5-[(diaminomethylidene)amino]-2-oxopentanoic acid | C6 H11 N3 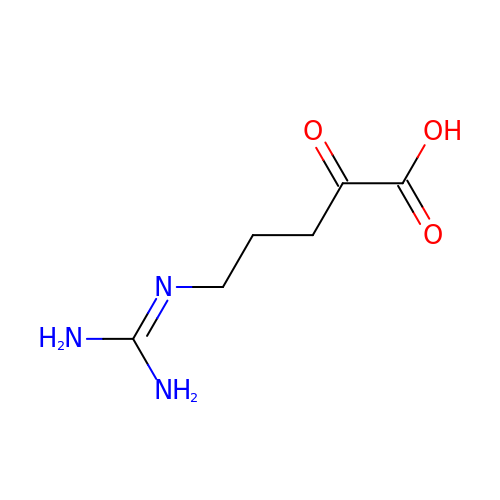O3 | ARBHXJXXVVHMET-UHFFFAOYSA-N ethyl 6-bromanyl-2-[(dimethylamino)methyl]-5-oxidanyl-1-phenyl-indole-3-carboxylate | C20 H21 Br 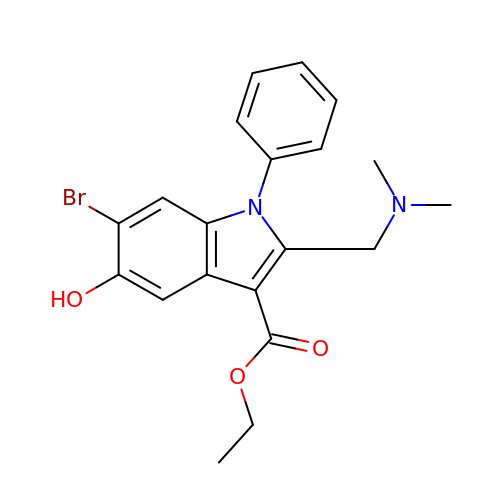N2 O3 | UJLZWNQHEVGZBY-UHFFFAOYSA-N Pectocin M1 and M2 consist of an M-class cytotoxic domain with lipid II degrading activity, fused to a plant-like ferredoxin domain (Grinter et al., 2012a; 2013,). This ferredoxin domain, which contains an intact [2Fe-2S] iron–sulphur cluster, substitutes for the helical receptor binding domain and IUTD of the M-class bacteriocins discussed above, that are required to deliver the cytotoxic domain to the periplasm. We have previously demonstrated that Pectobacterium spp. are able to acquire iron directly from plant ferredoxin under iron-limiting conditions through a receptor mediated process and that the bacteriocins pectocin M1 and M2 parasitize this system for cell entry through presentation of a ferredoxin domain (Grinter et al., 2013). The lack of an IUTD indicates that the ferredoxin-containing pectocins utilize an existing ferredoxin uptake mechanism to cross the OM, without direct interaction with the Tol or Ton complexes in the periplasm.

In initial crystallization trials for pectocin M2, characteristic red-brown crystals of this ferredoxin-containing bacteriocin formed with PEG 3350 and ammonium sulphate as the precipitants. Data from these crystals were collected to 2.3 Å in the space group P21 and phased using anomalous scattering data from the metal centres of the [2Fe-2S] iron–sulphur cluster. The structure of pectocin M2 revealed an N-terminal domain with the predicted ferredoxin-fold (residues 2–94, in red), separated from the colicin M-like cytotoxic domain (residues 116–271, in blue) by a linker region (residues 95–115, in green) that forms an α-helix. There is a significant difference in the orientation of the cytotoxic and ferredoxin domains of the two pectocin M2 molecules in the asymmetric unit (ASU) with a root mean square deviation (r.m.s.d.) of 3.4 Å, between main-chain atoms. The relative orientation of the ferredoxin domain, linker region and cytotoxic domain gives rise to a non-linear dog-leg structure. Mg2+, Ca2+ or Mn2+ ions are required for catalytic activity of M-class bacteriocins, and analysis of these proteins has shown co-ordination at this position to be essential for activity (Grinter et al., 2012b). In the pectocin M2 structure this key aspartate (D226) adopts an analogous conformation. However, no density for a metal ion is observed in this position, which is occupied by a water molecule. The observation that there is a relatively large difference in orientation between the cytotoxic and ferredoxin domains in the monomers of the ASU is suggestive of such flexibility and indicates that the crystal structure may not be wholly representative of pectocin M2 in solution.

>[2x]MATYKVKDVTTGAEIEVPDDKYILDEFEKQGVNLPYSCRAGACSSCVALISSGEVDQSDGSFLSEKQEKKYILTCCSYPKSDCTIETGYEDKILEDFEIELAETGLEFFNDLKDSLPRSGEILSGVTAPFEAFDHYLFGNGVERSININDVGFNINVSQIPPIMSLLNGKNVGRFDIGSDFVRNTALDGYSVAAYLGNITMRTEGVLNVKSDGTWQYEGVIRSYNDTYDANPSTHRGALGEWATGVLNNLSGTPYEIRIPGELKIKENGKKLEHHHHHH> RRRRRRR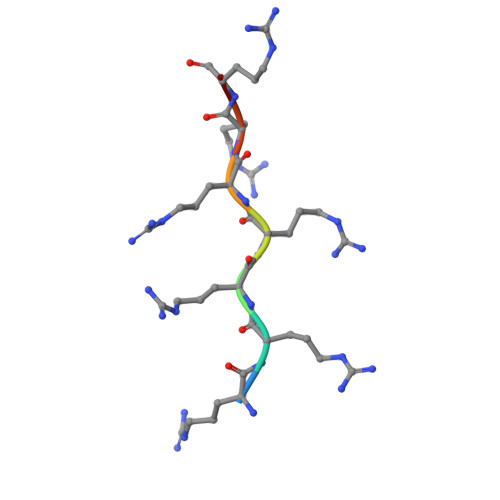R>GPGSGGSGVQTAYWVQEA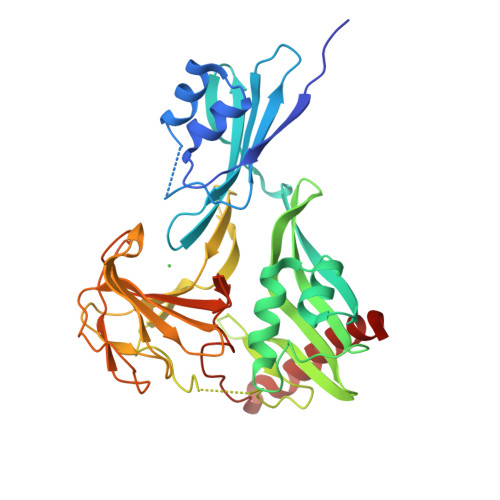VQPGDSLADVLARSGMARDEIARITEKYGGEADLRHLRADQSVHVLVGGDGGAREVQFFTDEDGERNLVALEKKGGIWRRSASEADMKVLPTLRSVVVKTSARGSLARAEVPVEIRESLSGIFAGRFSLDGLKEGDAVRLIYDSLYFHGQQVAAGDILAAEVVKGGTRHQAFYYRSDKEGGGGGNYYDEDGRVLQEKGGFNIEPLVYTRISSPFGYRMHPILHTWRLHTGIDYAAPQGTPVRASADGVITFKGRKGGYGNAVMIRHANGVETLYAHLSAFSQAQGNVRGGEVIGFVGSTGRSTGPHLHYEARINGQPVNPVSVALPTPELTQADKAAFAAQKQKADALLARLR[2x]>VSNAIKFIILTEIIFPTLLLVFGIYHGVMQVFYRSGIIKAESFLGIDYYQGLTLHGVINVIVYTTIFIVGFSNAIVAYSLKKPLREKVQWIALGMMVIGTLMAAWAMFTGRATVLYTFYPPLIAHWTFYLGAVLLVLGSLVPFFFDWIPSAIQWKRENPDQKLPLAVFGTFVNFILWTIMIVPVAIEILFQLLPLSLGLVDEINPLLARTLFWFFGHPVVYFWLLPAYVALYTILPKIVSEKGKLYSDPAARLAFILFLIFSLPVGLHHQFTDPGITNTWKLIHALFTFGVALPSMITAFTVATSLEYSVKAEHPELKNSKFYWWTFLPFMRLEGNKWMFSYFFAGLVLFFIGGITGIVNASYNVNLVVHNTAYVPGHFHTTVGGLVLLVFFALSLYMVSKLRGSEVKLKGLAVLAPYFWMQGMFMFSYAMMVGGVVVGFPRRTNAGLTYLNPDSPLYRPEWTGYAQLAAVGGVLLAIGFAFYFASLIATALAPKVRESTLEFPIADAYHDAPAPLLNNLKTWTVAAIILAVLSYIPPLYDASVRGVFFKSPAYNEKFPMPLKQLQGAEKKEEKKELSKAEGGITQK[2x];>[2x]RAEKTGLTLALILLLTFFSLIVYAAKGLKIDIPTCVTDVEPFQEGKLIKHGDKRYELHILARMWYFDFNKGATEIKIPVGSVVDIFTTSKDVVHGVH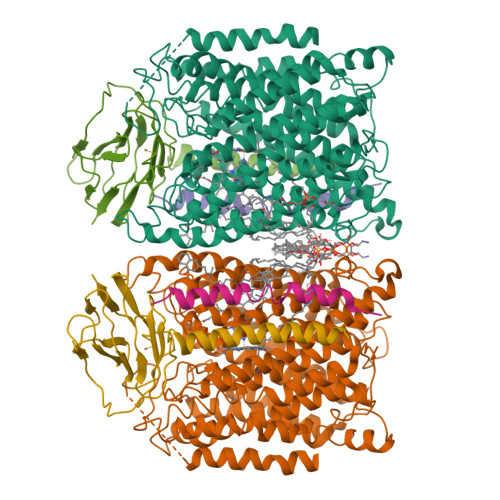IHGTNYNVMAIPGTVGYMRIKFEKPGVYHVVCHEFCGVGHHAMQGKIIVE;>[2x]FFPSGTIAFFIFMMVFYAVLWFMIYWVLLERG>[2x]MSSPEPPTEPPEPDNPTWSTQPTYSNLGQIRAHLLPSKACRLRTPGSLSTNPEPLPPPLPKKILTRTQSLPTRRTLHPSSIQVQPPRRPFLGSHSVDKSQAAVGPACLPAELTFGPADAPLGLSLRDLHSPEAVHTALAARQLQGLRTIYARLRARLMGGHPGPCHPGHSFRLLDSSPCAESGDALYYRVVRAHEDAWHILVAKVPKPGADVPHPWGLELQASLSPHFNLQGLCGLVPEGTLPGAPWRGAVALAAEVPERTVAQWLAEACTQPPEEFVWAVALLLLQLSAALKFLEAWGAALVELRPENLLLVAPRGCATTGPPRLLLTDFGRVCLQPPGPPGSPGPHAPQLGSLLRALLSLAAPSTTPLAAGLELLAAQLTRLRPSASRTRGALQALLWGPGPELRGRGAPLGPWLRALGPWLRVRRGLLVLRLAERAAGGEAPSLEDWLCCEYLAEATESSMGQALALLWDLEGGGGADYKDDDDKGPV

PEAK pseudokinases are molecular scaffolds which dimerize to regulate cell migration, morphology, and proliferation, as well as cancer progression. The pseudopodium-enriched atypical kinase (PEAK) family of pseudokinases, also known as New Kinase Family 3 (NKF3), is composed of three members: PEAK1 (also known as Sugen kinase [SgK] 269), PEAK2 (also known as Pragmin or SgK223), and PEAK3 (also known as chromosome 19 Open Reading Frame 35 [C19orf35]). Crystal structures of truncated PEAK1 and PEAK2 lacking the unstructured N-terminal domains revealed that these pseudokinase domain-flanking helices fold into an “XL”-shaped helical bundle and facilitate dimerization by forming an “XX”-shaped high-affinity dimerization interface termed the Split HElical Dimerization (SHED) domain. 14-3-3s are ubiquitous regulatory proteins that act as dimeric scaffolds to modulate their client proteins through a wide array of mechanisms, such as altering protein-protein interactions, inducing conformational changes, regulating subcellular localization, and sterically blocking access to phosphorylation sites.

We observed both PEAK3/14-3-3 complex and PEAK3 homodimer particles in the cryo-EM dataset; however, these particles exhibited orientation bias which limited our ability to reconstruct high-resolution maps. The addition of detergent to combat the orientation bias required us to work in a higher protein concentration regime, which shifted the particle equilibrium toward the complex, limiting the number of PEAK3-only particles. Nevertheless, the available PEAK3-only particles were initially processed in CryoSPARC and then re-extracted and imported to RELION for 3D classification and refinement to further alleviate streaking artifacts common for samples with preferred orientation. This yielded a low-resolution (4.9 Å) reconstruction of the PEAK3 homodimer. The limited resolution could be due to the low number of particles in the resulting reconstruction, especially impactful for a protein of this small size (108,034 Da). Another possibility is that the apo-PEAK3 homodimer exhibits conformational flexibility that is reduced upon 14-3-3 binding. Globally, however, comparison of the PEAK3/14-3-3 structure with the low-resolution structure of the PEAK3 homodimer alone did not reveal major differences within the PEAK3 dimer, with an overall average RMSD of 0.623 Å. The overall architecture of the PEAK3 pseudokinase homodimer within the PEAK3/14-3-3 complex, or alone solved at lower resolution, shows significant twisting between two pseudokinase domains instigated by rotations of the SHED domain helices, αJ and αL, relative to PEAK1 and PEAK2. These differences are thus independent from 14-3-3 binding and intrinsic to PEAK3.>MVLYFIGLGLYDERDITVKGLEIAKKCDYVFAEFYTSLMAGTTLGRIQKLIGKEIRVLSREDVELNFEKIVLPLAKENDVAFLTPGDPLVATTHAELRIRAKRAGVESYVIHAPSIYSAVGITGLHIYKFGKSATVAYPEGNWFPTSYYDVIKENAERGLHT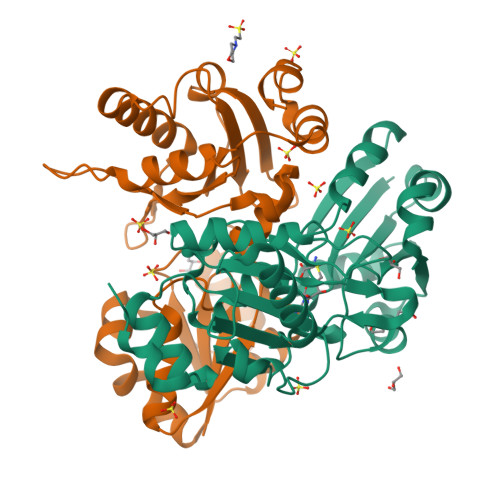LLFLDIKAEKRMYMTANEAMELLLKVEDMKKGGVFTDDTLVVVLARAGSLNPTIRAGYVKDLIREDFGDPPHILIVPGKLHIVEAEYLVEIAGAPREILRVNV[2x]> MDYIKGIAFDLYGTLFDVHSVVGRCDEAFPGRGREISALWRQKQLEYTWLRSLMNRYVNFQQATEDALRFTCRHLGLDLDARTRSTLCDAYLRLAPFSEVPDSLRELKRRGLKLAILSNGSPQSIDAVVSHAGLRDGF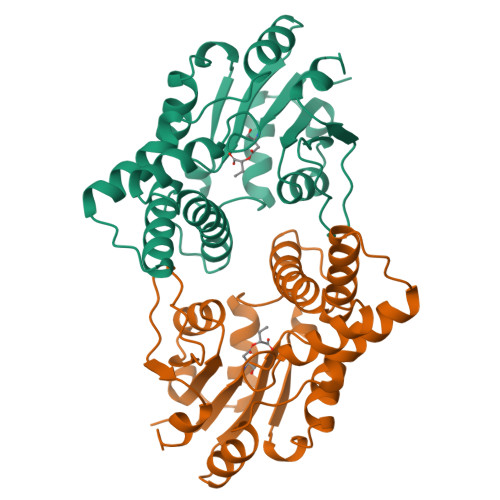DHLLSVDPVQVYKPDNRVYELAEQALGLDRSAILFVASNAWDATGARYFGFPTCWINRTGNVFEEMGQTPDWEVTSLRAVVELFETAAGKAEKG>MGQLIDGVWHDTWYDTKSTGGKFQRSASAFRNWLTADGAPGPTGTGGFIAEKDRYHLYVSLACPWAHRTLIMRKLKGLEPFISVSVVNPLMLENGWTFDDSFPGATGDTLY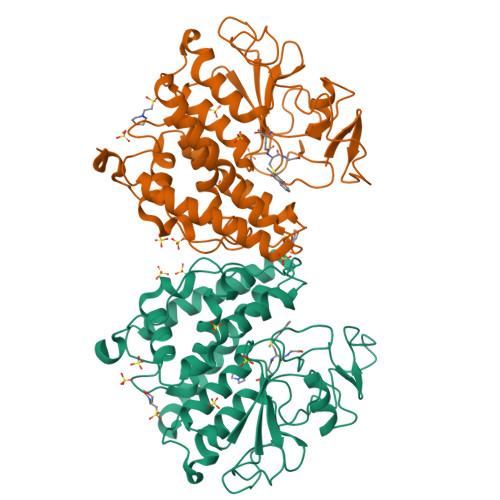QNEFLYQLYLHADPHYSGRVTVPVLWDKKNHTIVSNESAEIIRMFNTAFDALGAKAGDYYPPALQTKIDELNGWIYDTVNNGVYKAGFATSQEAYDEAVAKVFESLARLEQILGQHRYLTGNQLTEADIRLWTTLVRFDPVYVTHFKCDKHRISDYLNLYGFLRDIYQMPGIAETVNFDHIRNHYFRSHKTINPTGIISIGPWQDLDEPHGRDVRFG[2x]> TVGAVALDLDGNLAAATSTGGMTNKLPS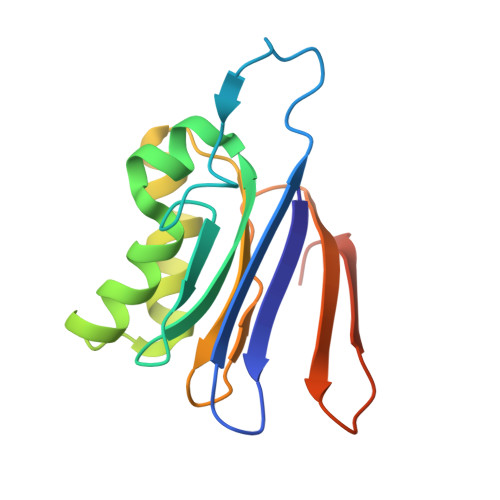TVGSSPLVGAGCYANNASVAVSCTGTGEVFIRALAAYDIAALMDYGGLSLAEACERVVMEKLPALGGSGGLIAIDHEGNVALPFNTEGMYRAWGYAGDTPTTGIYREKGDTVATQ2-(4-chlorophenyl)-4-[(3S)-piperidin-3-ylamino]thieno[3,2-c]pyridine-7-carboxamide 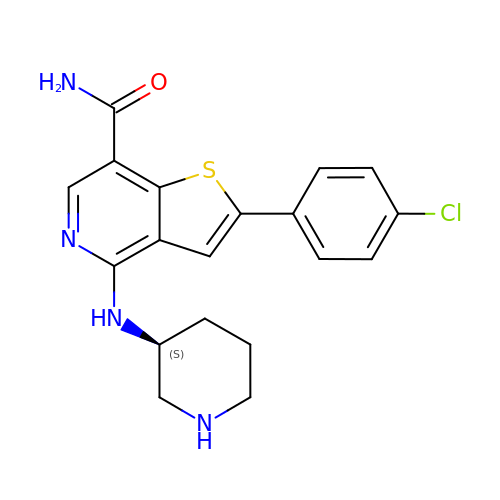| C19 H19 Cl N4 O S | QTBPGDBHORPJSA-ZDUSSCGKSA-N Finally, the CDPME2P is converted into MEcDP with concomitant release of CMP by MEcDP synthase (IspF). In this study, crystal structures of BsIspF in native and complexed with CMP have been determinated both at 1.99-Å resolutions. The monomer displays an α/β fold constructed with a four-strand β-sheet of β1, β2, β3, and β4, with β2 antiparallel to the others on one side, and a three-helix bundle of α1 to α3 on the other. In BsIspF trimer, the four-strand β-sheet of each subunit lay roughly parallel to the threefold NCS axis, forming a compact bell-shaped trimer of approximately 45 × 60 Å in the axial and equatorial dimensions, respectively.

The BsIspF crystallizes in space group P21, with unit-cell parameters a =56.96, b =89.30, c =84.71 Å, β =100.85°. The crystallographic asymmetric unit contains six monomers, which are arranged as two trimers of closely associated subunits. Overall, the two trimers are extremely similar with a root mean square deviation (r.m.s.d) value of 0.20 Å over all Cα atoms. The largest Cα r.m.s.d differences (~1.5 Å) between the two trimers occur in two loop regions, the first one connects β1 to α1 with the residues 34–39, and the second one links α1 to α2, which comprises residues 62–72. Both loops are parts of the active pocket and involved in the binding of 2-C-methyl-d-erythritol (MEPP) moiety. BsIspF trimer have three active pockets which are formed by the interface between two adjacent subunits, and here the magnesium ions deriving from the magnesium formate dehydrate used in crystallization are co-ordinated by the side chains of two histidines and an aspartate (Asp9, His11, and His43). However, although the accessible surface area (ASA) of a BsIspF monomer (7584 Å2) is nearly the same as ASA of EcIspF monomer (7681Å2), the ASA of the BsIspF trimer (17966 Å2), is larger than that of EcIspF trimer (16293 Å2), which demonstrates a looser packing of the subunits of BsIspF. Compared with the structure of EcIspF, there is also a hydrophobic cavity along the three-fold symmetry axis of BsIspF homotrimer. The volume of the cavity of BsIspF (1024Å3) is larger than that of EcIspF (718Å3), which is consistent with the looser packing of the subunits in BsIspF. In BsIspF, no ligand binding in the cavity is observed because no obviously continuous electron density is found here, and only a hollow cavity is presumed in both native and BsIspF/CMP complex, but regarding the highly conserved residues involved in the cavity formation between B. subtilis and E. coli and the size or dimension of the cavity in BsIspF, potential ligands of isoprenoid species could bind here.

>MFRIGQGFDVHQLVEGRPLIIGGIEIPYEKGLLGHSDADVLLHTVADACLGAVGEGDIGKHFPDTDPEFKDADSFKLLQHVWGIVKQKGYVLGNIDCTIIAQKPKMLPYIEDMRKRIAEGLEADVSQVNVKATTTEKLGFTGRAEGIAAQATVLIQKG[6x]>MESRVTPVAVIGMGCRLPGGINSPDKLWESLLRGDDLVTEIPPDRWDADDYYDPEPGVPGRSVSRWGGFLDDVAGFDAEFFGISEREATSIDPQQRLLLETSWEAIEHAGLDPASLAGSSTAVFTGLTHEDYLVLTTTAGGLASPYVVTGLNNSVASGRIAHTLGLHGPAMTFDTACSSGLMAVHLACRSLHDGEADLALAGGCAVLLEPHASVAASAQGMLSSTGRCHSFDADADGFVRSEGCAMVLLKRLPDALRDGNRIFAVVRGTATNQDGRTETLTMPSEDAQVAVYRAALAAAGVQPETVGVVEAHGTGTPIGDPIEYRSLARVYGAGTPCALGSAKSNMGHSTASAGTVGLIKAILSLRHGVVPPLLHFNRLPDELSDVETGLFVPQAVTPWPNGNDHTPKRVAVSSFGMSGTNVHAIV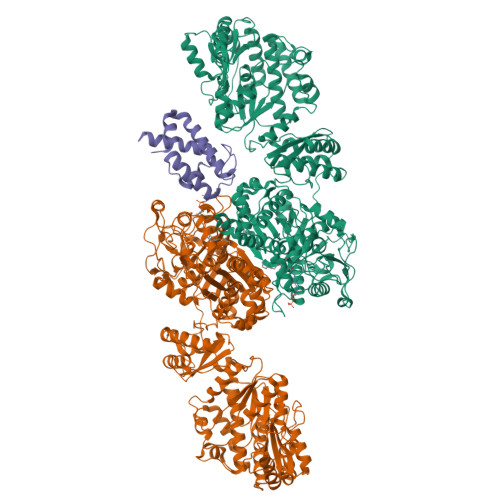EEAPAEASAPESSPGDAEVGPRLFMLSSTSSDALRQTARQLATWVEEHQDCVAASDLAYTLARGRAHRPVRTAVVAANLPELVEGLREVADGDALYDAAVGHGDRGPVWVFSGQGSQWAAMGTQLLASEPVFAATIAKLEPVIAAESGFSVTEAITAQQTVTGIDKVQPAVFAVQVALAATMEQTYGVRPGAVVGHSMGESAAAVVAGALSLEDAARVICRRSKLMTRIAGAGAMGSVELPAKQVNSELMARGIDDVVVSVVASPQSTVIGGTSDTVRDLIARWEQRDVMAREVAVDVASHSPQVDPILDDLAAALADIAPMTPKVPYYSATLFDPREQPVCDGAYWVDNLRNTVQFAAAVQAAMEDGYRVFAELSPHPLLTHAVEQTGRSLDMSVAALAGMRREQPLPHGLRGLLTELHRAGAALDYSALYPAGRLVDAPLPAWTHARLFIDDDGQEQRAQGACTITVHPLLGSHVRLTEEPERHVWQGDVGTSVLSWLSDHQVHNVAALPGAAYCEMALAAAAEVFGEAAEVRDITFEQMLLLDEQTPIDAVASIDAPGVVNFTVETNRDGETTRHATAALRAAEDDCPPPGYDITALLQAHPHAVNGTAMRESFAERGVTLGAAFGGLTTAHTAEAGAATVLAEVALPASIRFQQGAYRIHPALLDACFQSVGAGVQAGTATGGLLLPLGVRSLRAYGPTRNARYCYTRLTKAFNDGTRGGEADLDVLDEHGTVLLAVRGLRMGTGTSERDERDRLVSERLLTLGWQQRALPEVGDGEAGSWLLIDTSNAVDTPDMLASTLTDALKSHGPQGTECASLSWSVQDTPPNDQAGLEKLGSQLRGRDGVVIVYGPRVGDPDEHSLLAGREQVRHLVRITRELAEFEGELPRLFVVTRQAQIVKPHDSGERANLEQAGLRGLLRVISSEHPMLRTTLIDVDEHTDVERVAQQLLSGSEEDETAWRNGDWYVARLTPSPLGHEERRTAVLDPDHDGMRVQVRRPGDLQTLEFVASDRVPPGPGQIEVAVSMSSINFADVLIAFGRFPIIDDREPQLGMDFVGVVTAVGEGVTGHQVGDRVGGFSEGGCWRTFLTCDANLAVTLPPGLTDEQAITAATAHATAWYGLNDLAQIKAGDKVLIHSATGGVGQAAISIARAKGAEIFATAGNPAKRAMLRDMGVEHVYDSRSVEFAEQIRRDTDGYGVDIVLNSLTGAAQRAGLELLAFGGRFVEIGKADVYGNTRLGLFPFRRGLTFYYLDLALMSVTQPDRVRELLATVFKLTADGVLTAPQCTHYPLAEAADAIRAMSNAEHTGKLVLDVPRSGRRSVAVTPEQAPLYRRDGSYIITGGLGGLGLFFASKLAAAGCGRIVLTARSQPNPKARQTIEGLRAAGADIVVECGNIAEPDTADRLVSAATATGLPLRGVLHSAAVVEDATLTNITDELIDRDWSPKVFGSWNLHRATLGQPLDWFCLFSSGAALLGSPGQGAYAAANSWVDVFAHWRRAQGLPVSAIAWGAWGEVGRATFLAEGGEIMITPEEGAYAFETLVRHDRAYSGYIPILGAPWLADLVRRSPWGEMFASTGQRSRGPSKFRMELLSLPQDEWAGRLRRLLVEQASVILRRTIDADRSFIEYGLDSLGMLEMRTHVETETGIRLTPKVIATNNTARALAQYLADTLAEEQAAAPAASKLAAALEHHHHHH[3x]>[2x]AGVPGFPLPSIHTQQAYDP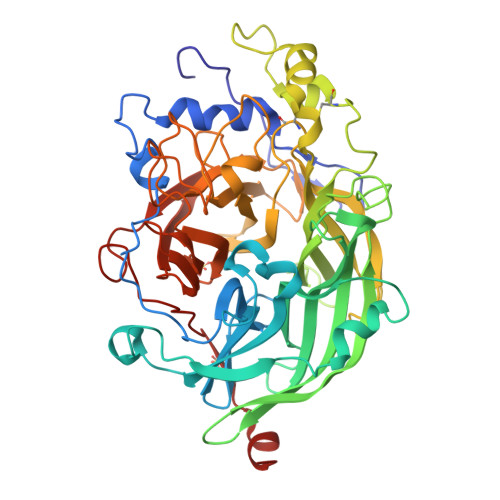QSDFTARWTRADALQIKAHSDATVAAGQNSLPAQLTMPNIPADFPVINPDVWVWDTWTLIDKHADQFSYNGWEVIFCLTADPNAGYGFDDRHVHARIGFFYRRAGIPASRRPVNGGWTYGGHLFPDGASAQVYAGQTYTNQAEWSGSSRLMQIHGNTVSVFYTDVAFNRDANANNITPPQAIITQTLGRIHADFNHVWFTGFTAHTPLLQPDGVLYQNGAQNEFFNFRDPFTFEDPKHPGVNYMVFEGNTAGQRGVANCTEADLGFRPNDPNAETLQEVLDSGAYYQKANIGLAIATDSTLSKWKFLSPLISANCVNDQTERPQVYLHNGKYYIFTISHRTTFAAGVDGPDGVYGFVGDGIRSDFQPMNYGSGLTMGNPTDLNTAAGTDFDPSPDQNPRAFQSYSHYVMPGGLVESFIDTVENRRGGTLAPTVRVRIAQNASAVDLRYGNGGLGGYGDIPANRADVNIAGFIQD8-(4-beta-D-glucopyranuronosylpiperazin-1-yl)-5-(morpholin-4-yl)-1,2,3,4-tetrahydro[1,2,3]triazino[4',5':4,5]thieno[2,3-c]isoquinoline | C26 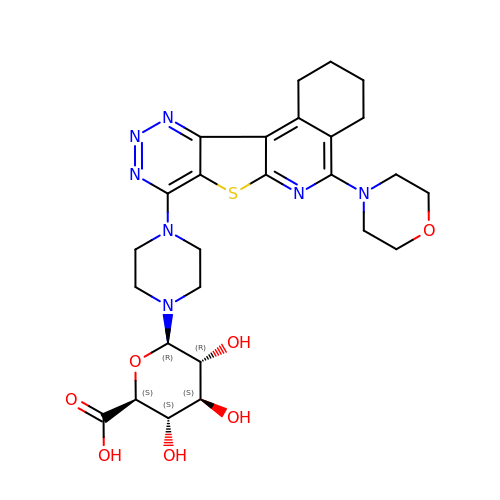H33 N7 O7 S | AQRGEQSNANJABA-WFFUTXBBSA-N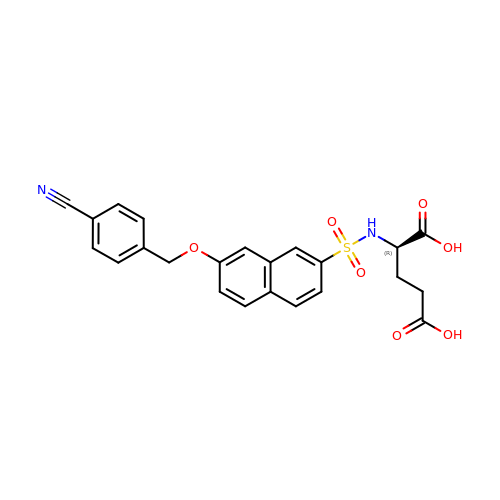N-({7-[(4-cyanobenzyl)oxy]naphthalen-2-yl}sulfonyl)-D-glutamic acid | C23 H20 N2 O7 S | DRAFRFXITJJMML-OAQYLSRUSA-N>MSPSIDVKSPDTSAGPLTIDGIADLRAKSAPIPTGVAPGTSSDMFKSPSCYTKPKAKRWDHYLSEESKSRQQSTLKGAARYLKTPGLISLGGGLPSPEYFPFEEISVKVPTPPGFSPHETQESGAVLTAKKGDVQAGRSLYDLEVALNYGQSTGSPQLLRFVTEHTELIHNPPYADWQCCLNAGSTYGWDTVLRMLCTRGDYILMEEYTFSSAKETALPLGVKVASVKMDAEGLLPESLDEVLSNWDEASRGSRKPFVLYTIPTGQNPTGATQQLERRKAVYKVAQKHDL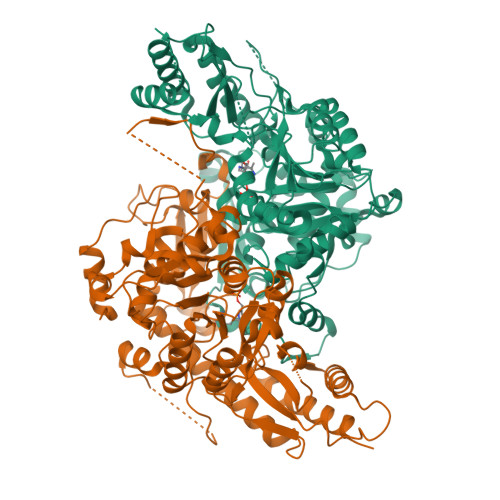IIVEDEPYYFLQMQPYTGPDREPVPPPASHDEFIKSLIPSYLSLDVDGRVLRLESFSKVLSPGSRTGWIVGPEQLVERFMRNCETGAQHPSGISQIVLFKLLDEHWGHSGYLDWLINLRMQYTGRRDAIVNACEKYLPKEIAKWNPPAAGMFHWIEIDWQKHPAVASGKSREAIEEAVFHAAVNNGVLVSRGSWFTAAGHNEGNLFFRATFAAASSENIAEAIARFATALRTEFSLLEHHHHHH[4x]> APADNTVNIKTFDKVKNAFGDGLSQSAEGTFTFPADVTTVKTIKMFIKNECPNKTCDEWDRYANVYVKNKTTGEWYEIGRFITPYWVGTEKLPRGLEIDVTDFKSLLSGNTELKIYT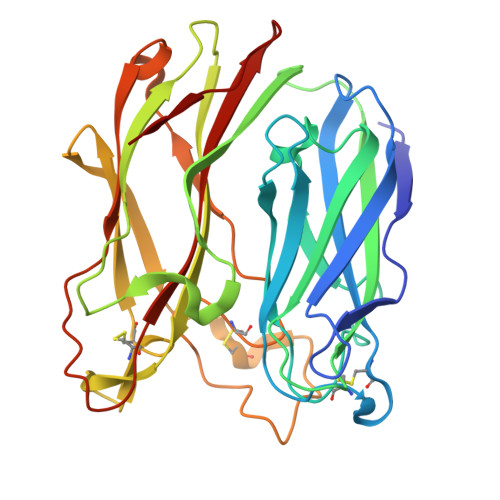ETWLAKGREYSVDFDIVYGTPDYKYSAVVPVIQYNKSSIDGVPYGKAHTLGLKKNIQLPTNTEKAYLRTTISGWGHAKPYDAGSRGCAEWCFRTHTIAINNANTFQHQLGALGCSANPINNQSPGNWTPDRAGWCPGMAVPTRIDVLNNSLTGSTFSYEYKFQSWTNNGTNGDAFYAISSFVIAKSNTPISAPVVTN>GSGLDDVSNKAYEDAEAKAKYEAEAAFFANLKLSDFNIIDTLGVGGFGRVELVQLKSEESKTFAMKILKKRHIVDTRQQEHIRSEKQIMQGAHSDFIVRLYRTFKDSKYLYMLMEACLGGELWTILRDRGSFEDSTTRFYTACVVEAFAYLHSKGIIYRDLKPENLILDHRGYAKLVDFGFAKKIGFGKKTWTFCGTPEYVAPEIILNKGHDISADYWSLGILMYELLTGSPPFSGPDPMKTYNIILRGIDMIEFPKKIAKN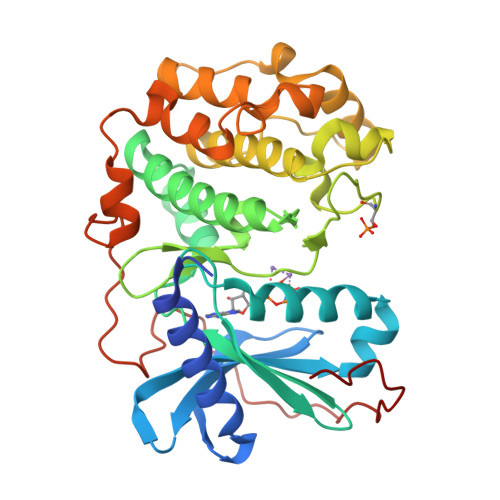AANLIKKLCRDNPSERLGNLKNGVKDIQKHKWFEGFNWEGLRKGTLTPPIIPSVASPTDTSNFDSFPEDNDEPPPDDNSGWDIDF[4x]>MSLTDAKIRTLKPSDKPFKVSDSHGLYLLV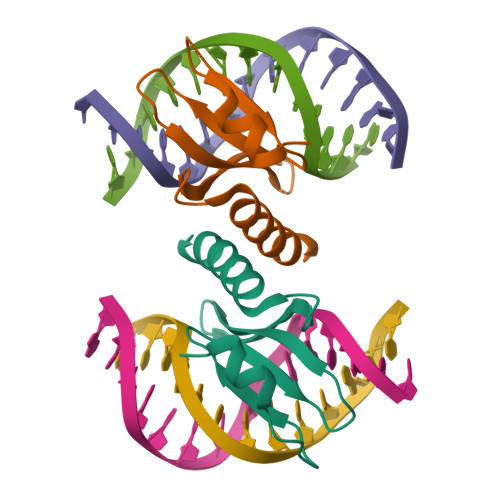KPGGSRHWYLKYRISGKESRIALGAYPAISLSDARQQREGIRKMLALNINLEHHHHHH[2x]>GLSKEQESIIKLAENGHNIFYTGSAGTGKSILLREMIKVLKGIYGRENVAVTASTGLAACNIGGITIHSFAGIGLGKGDADKLYKKVRRSRKHLRRWENIGALVVDEISMLDAELLDKLDFIARKIRKNHQPFGGIQLIFCGDFFQLPPVSKDPNRPTKFAFESKAWKEGVKMTIMLQKVFRQRGDVKFIDMLNRMRLGNIDDETEREFKKLSRPLPDDEIIPAELYSTRMEVERANNSRLSKLPGQVHIFNAIDGGALEDEELKERLLQNFLAPKELHLKVGAQVMMVKNLDATLVNGSLGKVIEFMDPETYFCYEALTNDPSMPPEKLETWAENPSKLKAAMEREQSDGEE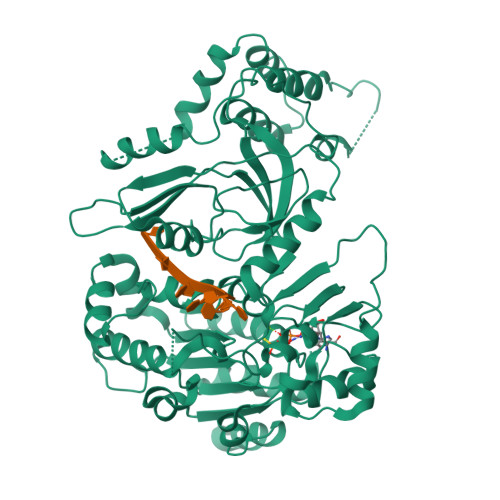SAVASRKSSVKEGFAKSDIGEPVSPLDSSVFDFMKRVKTDDEVVLENIKRKEQLMQTIHQNSAGKRRLPLVRFKASDMSTRMVLVEPEDWAIEDENEKPLVSRVQLPLMLAWSLSIHKSQGQTLPKVKVDLRRVFEKGQAYVALSRAVSREGLQVLNFDRTRIKAHQKVIDFYLTLSSAESAYKQLEADEQV[2x]>[2x]MAEEGTRSEAADAATQARQLPDSRNIFVSHRFPERQVDLGEVVMNFAEAGSPDNPALLLLPEQTGSWWSYEPVMGLLAENFHVFAVDIRGQGRSTWTPRRYSLDNFGNDLVRFIALVIKRPVVVAGNSSGGLLAAWLSAYAMPGQIRAALCEDAPFFASELVPAYGHSVLQAAGPAFELYRDFLGDQWSIGDWKGFVEAAKASPAKAMQLFPTPDEAPQNLKEYDPEWGRAFFEGTVALHCPHDRMLSQVKTPILITHHARTIDPETGELLGALSDLQAEHAQDIIRSAGVRVDYQSHPDALHMMHLFDPARYAEILTSWSATLPANDHHHHHH

Zearalenone (ZEN) is a mycoestrogenic polyketide produced by Fusarium graminearum and other phytopathogenic members of the genus Fusarium. ZenA cleaves zearalenone [ZEN, (S,E)-14,16-dihydroxy-3-methyl-3,4,5,6,9,10-hexahydro-1H-benzo[c][1]oxacyclotetradecine-1,7(8H)-dione] to hydrolyzed zearalenone [HZEN, (S,E)-2,4-dihydroxy-6-(10-hydroxy-6-oxoundec-1-en-1-yl)benzoic acid], which decarboxylates spontaneously to decarboxylated hydrolyzed zearalenone [DHZEN, (S,E)-1-(3,5-dihydroxyphenyl)-10-hydroxyundec-1-en-6-one]. Furthermore, we report site-directed mutagenesis as well as structural analysis of the dimeric ZenARe of R. erythropolis and the more thermostable, tetrameric ZenAScfl of Streptomyces coelicoflavus with and without bound ligands. The X-ray crystal structures not only revealed canonical features of α/β hydrolases with a cap domain including a Ser-His-Asp catalytic triad but also unusual features including an uncommon oxyanion hole motif and a peripheral, short antiparallel β-sheet involved in tetramer interactions.

As inactivation of ZenAScfl by substituting the catalytic His-286 with tyrosine (H286Y) caused conformational changes at the active site, we attempted to get structural information with a bound, noncleavable substrate analogue. A derivative of ZEN, which is a cyclic amide rather than a cyclic carboxylic ester, was synthesized. In line with proposed nomenclature guidelines, we called the molecule zearalactamenone (ZLAEN). The ligand was found at the active site of ZenARe, and the resorcylic acid moiety was in the same position as the one of HZEN in ZenAScfl H286Y. Most of the structure of ZenARe remained unchanged upon binding of ZLAEN. However, the positions of the amino acids Met-208 – Pro-214 at the lip of the cap were shifted upon binding. The biggest movements were observed for Leu-210, where Cα was shifted by 4.4 Å and CD by 6.7 Å, and Phe-211, where the Cα was shifted by 3.1 Å, and side-chain atoms were shifted by up to 5.8 Å. The nucleophilic Ser-112 appeared in the same orientation as in the unbound structure, forming a hydrogen bond with N21 of ZLAEN at a distance of 3.5 Å. The side-chain amide of Gln-63 formed a hydrogen bond of 2.8 Å with the hydroxyl group connected to C-16 of ZLAEN. However, crystal structure analysis revealed that only ZenARe underwent a structural change resembling enzyme closure, with residues in the cap’s lip adopting a more closed conformation of the ZEN-binding pocket.The cGMP-dependent protein kinases (PKG) belong to the family of serine/threonine kinases and are one of the major intracellular receptors for cGMP. Next, two cyclic-nucleotide binding domains (CNBD-A and CNBD-B) are followed by the catalytic domain. Binding of cGMP to the CNBDs is thought to induce a conformational change that activates the kinase by removing the autoinhibitory domain from the catalytic cleft, leaving the catalytic domain free to phosphorylate downstream substrates. To understand the overall architecture of the cGMP-binding domain and the molecular features required for cGMP binding, we determined crystal structures of the CNBD-A of human PKG I bound to cGMP, cAMP or in the absence of bound nucleotide.

To gain additional insight into cyclic-nucleotide binding specificity, we determined the crystal structure of CNBD-A in the presence of cAMP. Despite its unique crystallization buffer conditions, the PKG Iβ:cAMP complex showed similar crystal parameters and contacts as the PKG Iβ:cGMP complex containing two molecules in the unit cell. cAMP:A is similarly located at the interface between the two molecules, but makes no hydrogen bonds with molecule B. A surprising feature of the PKG Iβ (92–227):cAMP complex is that cAMP binds in two different conformations, anti in one molecule and syn in the other. While the sugar phosphates share the same set of contacts with the protein as the PKG Iβ:cGMP complex at site 1, each purine ring of cAMP shows different contacts with the protein at sites 2 and 3, depending on its orientation. For example, the hydroxyl group of Thr193 at site 2 interacts with the unprotonated nitrogen at the 2-position through a weak hydrogen bond for the syn-configured cAMP whereas no such contact exists in the anti-configured cAMP. Cys173, makes a hydrogen bond with the unprotonated N7 of the syn-configured cAMP, whose distance is 3.6 Å, but no such contact exists for cAMP in the anti conformation. The side chains of Val165 and Met175 near site 3 come within 3.5–3.8 Å of the purine ring for syn-configured cAMP, but they are beyond van der Waals distance for anti-configured cAMP. Superposition of the two molecules at the PBC reveals that the differences in cAMP binding are mainly caused by the β4 and β5 strands moving away from the PBC to accommodate the extended conformation of the anti-configured cAMP (Fig. middle panel on Fig. 5C). In contrast, the structure with anti-configured cAMP shows the highest B-factors at this region, indicating that site 3 residues do not interact as strongly with the adenine ring. While the PKG Iβ:cAMP complex was crystallized in the same P6222 space group, with similar crystal parameters and contacts, cAMP:A does not form hydrogen bonds with molecule B and PBC:B shows no apparent contact induced structural changes. Since a hydrogen atom replaces the 2-NH2 group in cAMP, no such interaction is possible, and cAMP binds the PKG CNBD-A in both syn- or anti-configurations.

>GSGSHVTLPFYPKSPQSKDLIKEAILDNDFMKNLELSQIQEIVDCMYPVEYGKDSCIIKEGDVGSLVYVMEDGKVEVTKEGVKLCTMGPGKVFGELAILYNCTRTATVKTLVNVKLWAIDRQCFQTIMMRTGLIKHTEY[2x]> 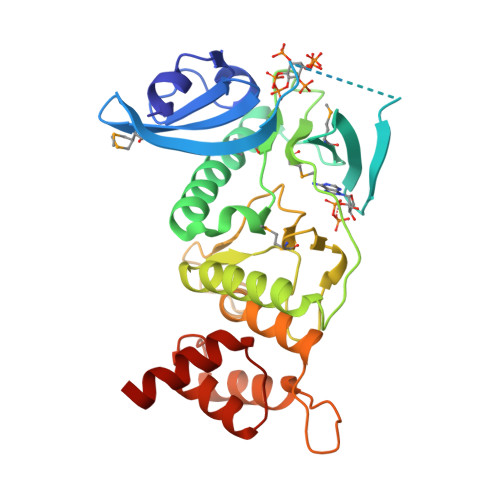AMPKINKIVNGTDLTPHYLSEPNKEFKIYRYNNEVYAVRFENDEPMDYVLMWKSHKSEHTQNSEMIKNTEEDYKELGKGEQGTVYEKTEDKAMKVSRGRHPREFYEEINLHIIEQQFFLKYHGIQEHFVLGLWNIKNEENVYFYMPKINAIPINKKIDQPKIEEFVLALKELNDAGYWHPDLANNPYHISPQNLIATEEMVKTIDLDGGFRYDKGRVDELSRKSLVYGKDQWLYVYNFIYPPTDEEDHRIDWRVPIEKWYENNRDESLSDNPHTLLRFYHEGLISLPKKLAHDLHETILEEL> FPTIPLSRLFDNAMLRAHRLHQLAFDTYQEFEEAYIPKEQKYSFLQNPQTSLCFSESIPTPSNREETQQKSNLELLRISLLLIQSWLEPVQFLRSVFAN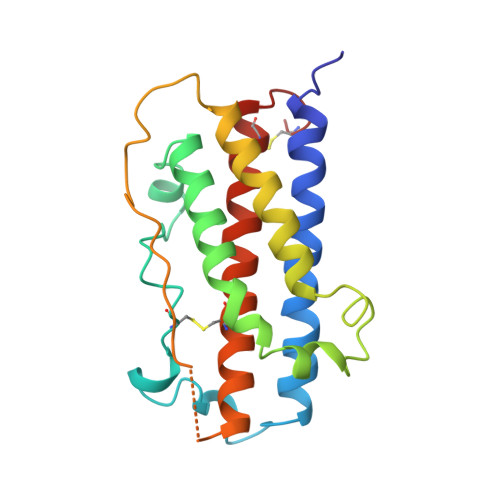SLVYGASDSNVYDLLKDLEERIQTLMGRLEDGSPRTGQIFKQTYSKFDTNSHNDDALLKNYGLLYCFRKDMDKVETFLRIVQCRSVEGSCGF>[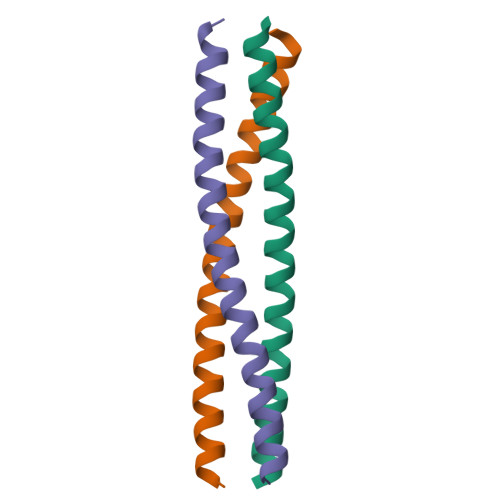5x]SQQQIAALSESLQATQQQLQALQQQCYELEKTNRLLVSEVMTLQKMVKAQ(5-amino-1H-1,2,4-triazol-1-yl)(4-methoxyphenyl)methanone | C10 H10 N4 O2 | 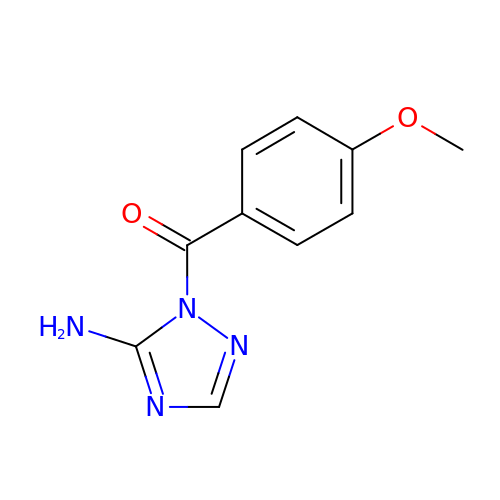MDFWUVGMSOBSKJ-UHFFFAOYSA-N> MSICPHIQQVFQNEKSKDGVLKTCNAAR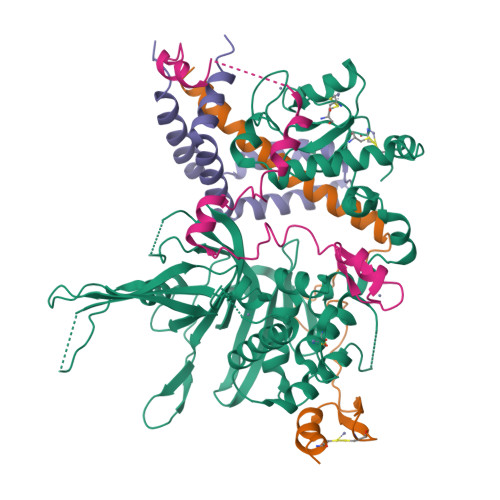YILNHSVPKEKFLNTMKCGTCHEINSGATFMCLQCGFCGCWNHSHFLSHSKQIGHIFGINSNNGLLFCFKCEDYIGNIDLINDAILAKYWDDVCTKTMVPSMERRDGLSGLINMGSTCFMSSILQCLIHNPYFIRHSMSQIHSNNCKVRSPDKCFSCALDKIVHELYGALNTKQASSSSTSTNRQTGFIYLLTCAWKINQNLAGYSQQDAHEFWQFIINQIHQSYVLDLPNAKEVSRANNKQCECIVHTVFEGSLESSIVCPGCQNNSKTTIDPFLDLSLDIKDKKKLYECLDSFHKKEQLKDFNYHCGECNSTQDAIKQLGIHKLPSVLVLQLKRFEHLLNGSNRKLDDFIEFPTYLNMKNYCSTKEKDKHSENGKVPDIIYELIGIVSHKGTVNEGHYIAFCKISGGQWFKFNDSMVSSISQEEVLKEQAYLLFYTIRQVN;> MTEETITIDSISNGILNNLLTTLIQDIVARETTQQQLLKTRYPDLRSYYFDPNGSLDINGLQKQQESSQYIHCENCGRDVSANRLAAHLQRCLSRGARR;> MTMDTAQLKSQIQQYLVESGNYELISNELKARLLQEGWVDKVKDLTKSEMNINESTNFTQILSTVEPKALEMVSDSTRETVLKQIREFLEEIVDTQ;> MRSGDAEIKGIKPKVIEEYSLSQGSGPSNDSWKSLMSSAKDTPLQYDHMNRESLKKYFNPNAQLIEDPLDKPIQYRVCEKCGKPLALTAIVDHLENHCAGASGK> MPEDILVDIKRDYVLSKLRDNERIDGRGFDEFRKVEIIPNVIEKAEGSALVKLGDTQVVVGVKMQPGEPYP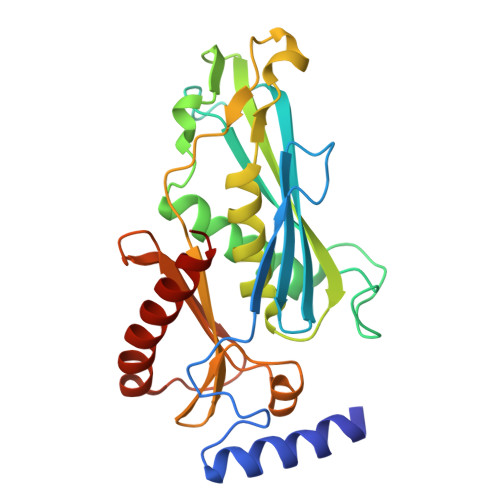DTPDRGVIIVNAELVPLASPTFEPGPPDENSIELARVVDRGIRESEAVDLSKLVIEEGEKVWIVFVDIHALDDDGNLLDASALAAIAALMNTKVPAERFDLGEDYLLPVRDLPVSVTSLIVGNKYLVDPSREEMSVGDTTLTITTDKDDNVVAMQKSGGYLLDEKLFDELLDVSINCARKLREKFKEI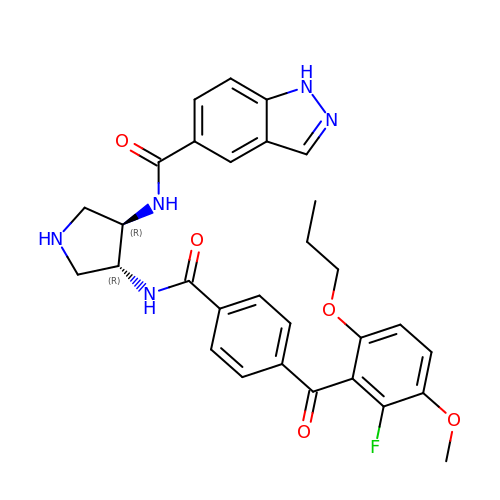N-[(3R,4R)-4-{[4-(2-fluoro-3-methoxy-6-propoxybenzene-1-carbonyl)benzene-1-carbonyl]amino}pyrrolidin-3-yl]-1H-indazole-5-carboxamide | C30 H30 F N5 O5 | AYXNTJKOINXKAJ-DHIUTWEWSA-N> SGDTDEPIFGKKPRIEESITEDLSLADLMPRVKVQSVETVEGCTHEVALPAEEDYLPLKPRVGKAAKEYPFILDAFQREAIQCVDNNQSVLVSAHTSAGKTVCAEYAIALALREKQRVIFTSPIKALSNQKYREMYEEFQDVGLMTGDVTINPTASCLVMTTEILRSMLYRGSEVMREVAWVIFDEIHYMRDSERGVVWEETIILLPDNVHYVFLSATIPNARQFAEWICHLHKQPCHVIYTDYRPTPLQHYIFPAGGDGLHLVVDENGDFREDNFNTAMQVLRDAGDLAKGDQKGRKGGTKGPSNVFKIVKMIMERNFQPVIIFSFSKKDCEAYALQMTKLDFNTDEEKKMVEEVFSNAIDCLSDEDKKLPQVEHVLPLLKRGIGIHHGGLLPILKETIEILFSE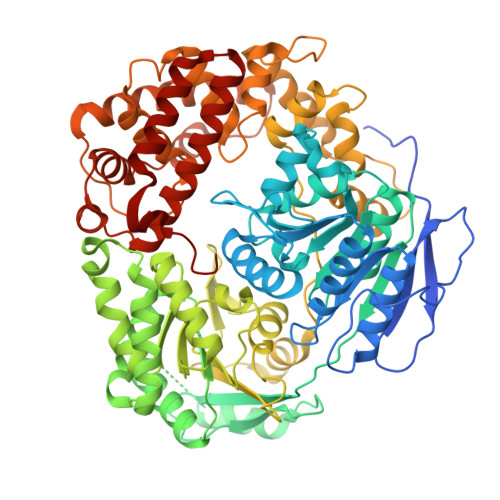GLIKALFATETFAMGINMPARTVLFTNARKFDGKDFRWISSGEYIQMSGRAGRRGMDDRGIVILMVDEKMSPTIGKQLLKGSADPLNSAFHLTYNMVLNLLRVEEINPEYMLEKSFYQFQHYRAIPGSRTVLQMDELKCRKRVLRRLGFATSSDVIEMKGRVACEISSADELLLTEMMFNGLFNDLSAEQATALLSCFVFQENSSEMPKLTEQLAGPLRQMQECAKRIAKVSAEAKLEIDEETYLSSFKPHLMDVVYTWATGATFAHICKMTDVFEGSIIRCMRRLEELLRQMCQAAKAIGNTELENKFAEGITKIKRDIVFAASLYL>MAPKSSSSGSKKKSSASSNSADAKASKFKLPAEFITRPHPSKDHGKETCTAYIHPNVLSSLEINPGSFCTVGKIGENGILVIARAGDEEVHPVNVITLSTTIRSVGNLILGDRLELKKAQVQPPYATKVTVGSLQGYNILECMEEKVIQKLLDDSGVIMPGMIFQNLKTKAGDESIDVVITDASDDSLPDVSQLDLNMDDMYGGLDNLFYLSPPFIFRKGSTHITFSKETQANRKYNLPEPLSYAAVGGLDKEIESLKSAIEIPLHQPTLFSSFGVSPPRGILLHGPPGTGKTMLLRVVANTSNAHVLTINGPSIVSKYLGETEAALRDIFNEARKYQPSIIFIDEIDSIAPNRANDDSGEVESRVVATLLTLMDGMGAAGKVVVIAATNRPNSVDPALRRPGRFDQEVEIGIPDVDARFDILTKQFSRMSSDRHVLDSEAIKYIASKTHGYVGADLTALCRESVMKTIQRGLGTDANIDKFSLKVTLKDVESAMVDIRPSAMREIFLEMPKVYWSDIGGQEELKTKMKEMIQLPLEASETFARLGISAPKGVLLYGPPGCSKTLTAKALATESGINFLAVKGPEIFNKYVGESERAIREIFRKARSAAPSIIFFDEIDALSPDRDGSSTSAANHVLTSLLNEIDGVEELKGVVIVAATNRPDEIDAALLRPGRLDRHIYVGPPDVNARLEILKKCTKKFNTEESGVDLHELADRTEGYSGAEVVLLCQEAGLAAIMEDLDVAKVELRHFEKAFKGIARGITPEMLSYYEEFALRSGSSS[6x]

The type II AAA + ATPase Drg1 is a ribosome assembly factor, functioning to release Rlp24 from the pre-60S particle just exported from nucleus, and its activity in can be inhibited by a drug molecule diazaborine. Here, we report Drg1 structures in different nucleotide-binding and benzo-diazaborine treated states. All structures display a typical three-layered architecture, similar to those of type II AAA + hexamers, such as p97/VCP and Cdc48, and the NTD, D1, and D2 rings show an apparent deviation from a perfect sixfold symmetry. Comparisons of these structures indicate that Drg1 hexamers transit between two extreme conformations, a planar and a helical state.

To obtain possible hybrid nucleotide bound states that best mimic the ATPase hydrolysis cycle of Drg1 and to illustrate the inhibition mechanism of benzo-diazaborine, we also incubated Drg1 with a mixture of ADP, AMPPNP, and benzo-diazaborine, as well as with a mixture of ATP and benzo-diazaborine. Taking the dataset of ADP/AMPPNP/benzo-diazaborine as an example, we performed deep 3D classification and analyzed the conformational differences between its planar and helical states. While the NTD and D1 rings are roughly superimposable, the D2 rings display a very large rotation between two states. While the six subunits in the planar or planar-like states are arranged more symmetrically, the subunits in the helical states adopt a spiral configuration to varying extents. Benzo-diazaborine was detected in the six D1 ATPase sites of the planar state, which is more symmetrical, whereas all the ATPase sites in the helical hexamer show no trace of benzo-diazaborine. Therefore, it is apparent that the treatment of Drg1 hexamers with benzo-diazaborine led to the formation of more symmetrical structures, indicating that the chemical also directly modulates the conformation of Drg1 hexamer, in addition to the inhibition of the ATP hydrolysis. The nucleotide binding to the D2 domains was only seen in structures from benzo-diazaborine treated samples, including the ADP/AMPPNP/benzo-diazaborine and ATP/benzo-diazaborine datasets. While the six D2 ATPase sites in the structure of the ATP/benzo-diazaborine dataset are fully occupied by ATP, the six D2 sites in the structures from the ADP/AMPPNP/benzo-diazaborine dataset are not saturated and appear to be partially occupied by ADP. In sharp contrast, in the protomer of planar benzo-diazaborine bound hexamer, the linker is in a loop conformation. Especially, M503 in the loop conformation is released from the hydrophobic interface.>MNTIAWLGRLVIERIRGIGVAALMLLQIIFSLPSAGGFGRFVYQMHRVGVMSLLIITVSGLFIGLVLGLQGYSILVNVGSESMLGTMVSLTLLRELAPVVAALLFAGRAGSALTAEIGSMKQSEQLASMEMIGVDPLKQIVSPRLWAGIVSLPMLTVIFAAIGIVGGKLVGVDFLGVDEGSFWSGMQNNVQFGHDVVNGIIKSIVFALLCTWIAVFQGYACDPTPEGIATAMTRTVVYSSLCVLGFDFVLTAVMFGGI[2x];>[2x]MMNNKTPLSTQSLIEVKNLSFNRGERVIYDNISLNIRRGQITAIMGPSGTGKTTLLRLIGGQLVPDQGEVLLDGKDIAQMSRQELFAARARMGMLFQSGALFTDMSVYENVAFPIRAHTKLSENLIAELVALKLESVGLRGTEQLMPTELSGGMNRRVALARAIALDPDLIMYDEPFAGQDPIVKGVLTRLIRSLREALDLTTIIVSHDVPETLSIADYIYVVAEGKIQGEGTPEELQAYASPFVKQFLTGSAEGPVEYQFSHQAYLDNEVRP;>VVQYLNQELVVSGKIDFENAEQ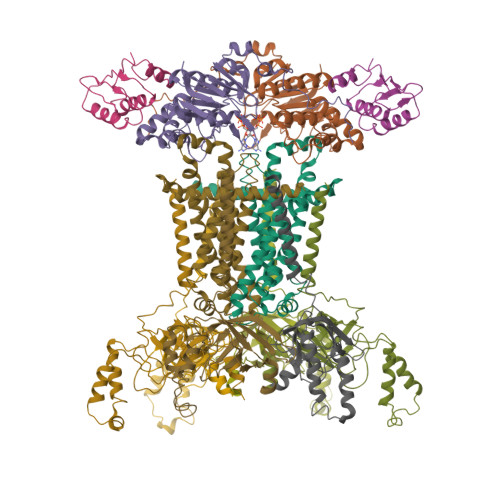QYQAGLAIIKKQTSFPLIVDLKQLEHGNTLALAVLVQWLRQTPQKSGLHFKNVPEKMLKIIQACHLQEDLHLVLEHHHHHH[2x];>MKSRTSELAVGIFVIIFGIALFFLAMKVSGLVGTNLSDGYTMKAQFDNVNGLKPRAKVTMSGVTIGRVDSITLDPVTRLATVTFDLDGKLTSFNAEQLKEVQKNALDELRYSSDYTQATPAQQKTMEQQLISNMNSITSIDEDAYIMVATNGLLGEKYLKIVPGGGLNYLKRGDTISNTQGTMDLEDLISKFITGGGAGKVAAGSSSAEEKAPASTDSSAQPSFVE[6x]>[2x]MPELPDFFEGKHF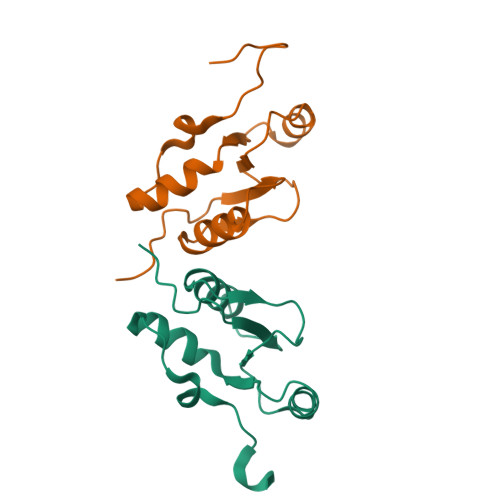FLYGEFPGDERRRLIRYVTAFNGELEDYMNERVQFVITAQEWDPNFEEALMENPSLAFVRPRWIYSCNEKQKLLPHQLYGVVPQAHHHHHH> MFRLTAASQKNLNSWYTKGTMRGGVPRIYYAWMRPGSFTRRRFEKMRNPFVDLETGTSLYFRDTRDSAEAIAHAADSKGIKGMDNAIDLYNEYRIVPDLYPEGFQWKHKLNTEYNQWRSNTWLTPDLIPKEHRGRFLCNFQLNIVAYDMRVV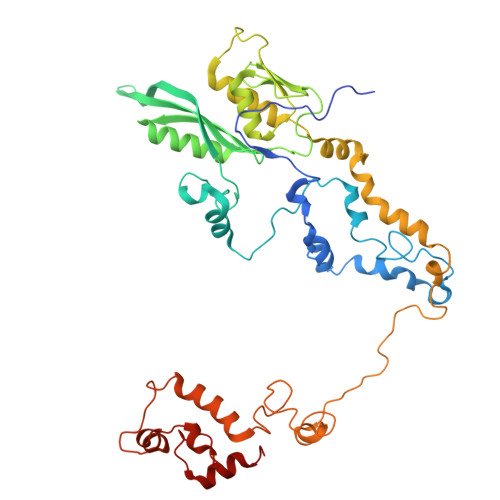KFSPKDHRQWIYCVLYVGSGKGIAGWGRAVAPSTQEAKKEAIREAFSNIIAVDLEQEGPMYPVRVNADGVRVLLYPARRIVANFRVADILCAFGFQHAGCRINLKATNNPKSPTHTVEGVFEAVKALRSVSEIAASRGKVPHSLIYNIYPYLEEIRRRKGMMAMHPPGKDGLLMPDRVVDNRLPDHLKRGYYDDVYWKDFFAGSDEHLNEPRMGLRGDEMRRRLEEAQTSPAPTTAKDTRRRTLEDVLKRLGKTTRDLGSIPIVNPRVDVGLPTHIKRNYQLH>[3x]MEASRLLLLLLLPLLLLFCNSVAAACSCTDSCSDAKESESKCGCKHEEETKQLPRSCKEIKLKTKTKEDGVYCLQTKSG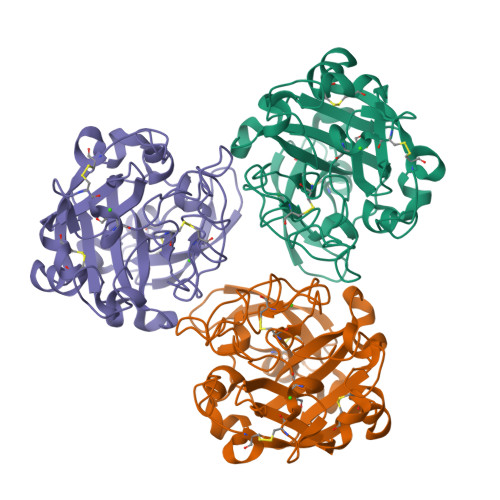QFYQAFCDMNTNGGGWTLVASVHENNIAAKCAIGDRWSSQLGSNPAVGFVDGDRSWANLNTFGRVESATDDDYKNPGYFDVDAEDISVWHVPNGTPLAQWKISSIFRYHTATEFLTPLGGNLYFLYKIFYPLVYGSGTCPASNGPAIPIVYDFGNTISVASQVCPACLGGTLQGYVHLRVFNNERAPFALCSGLRVLDNCNTEHYCIGGAGYVPEQTPRQCGDFSAFDWSGIGTHVEWSASKSLLEAAVFIFYR>[2x]TQDRPLLAVQEALKKCFPVVEEQQGLWQSALRDCQPLLSSLSNLAEQLQAAQNLRFEDV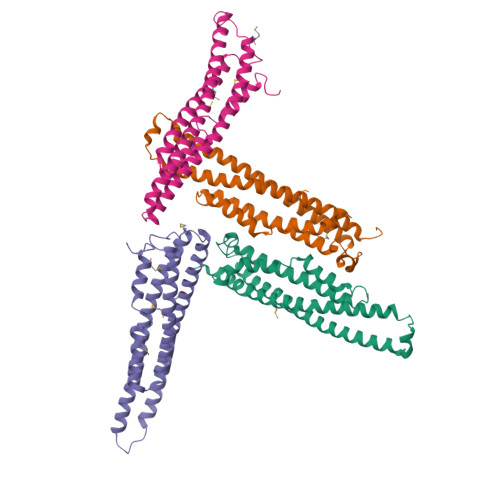PALRAFPDLKERLRRKQLVAGDIVLDKLGERLAILLKVRDMVSSHVERVFQIYEQHADTVGIDAVLQPSAVSPSVADMLEWLQDIERHYRKSYLKRKYLLSSIQWGDLANIQALPKAWDRISKDEHQDLVQDILLNVSFFLEE;>[2x]MVSARKIKDNAADWHNLILKWETLNDAGFTTANNIANLKISLLNKDKIELDSSSPASKENEEKVCLEYNEELEKLCEELQATLDGLTKIQVKMEKLSSTTKGICELENYHYGEESKRPPLFHTWPTTHFYEVSHKLLEMYRKELLLKRTVAKELAHTGDPDLTLSYLSMWLHQPYVESDSRLHLESMLLETGHRAL[(3~{S})-1-methyl-1-azoniabicyclo[2.2.2]octan-3-yl] 2-oxidanyl-2,2-diphenyl-ethanoate | C22 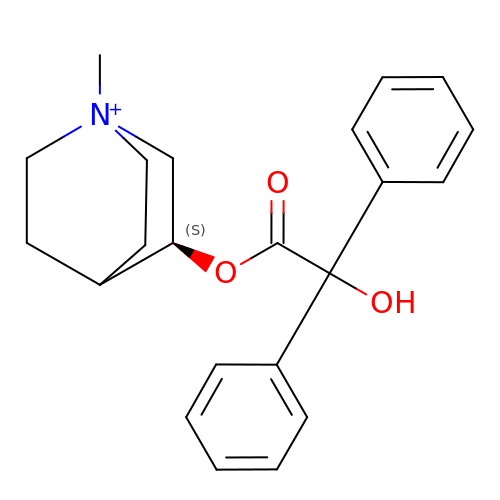H26 N O3 | HOOSGZJRQIVJSZ-LLBVYWAGSA-N>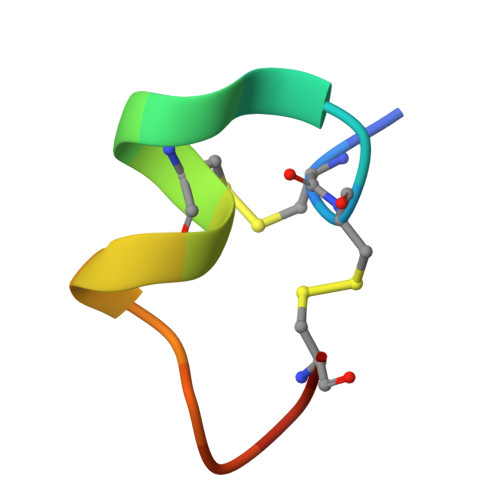 GCCSLPPCAANNPDYCX> SSLISKTIKYDPAKDKLITLASGSFWGTEHMYRKYLNDRIVDSKVGYANGEESKKDSPSSVSYKRVSGGDTDFAEVLQVSYNPKVITLRELTDFFFRIHDPTTSNSQGPDKGTQYRSGLFAHSDADLKELAKIKEEWQPKWGNKIATVIEPIKNFYDAEEYHQLYLDKNPQGYACPTH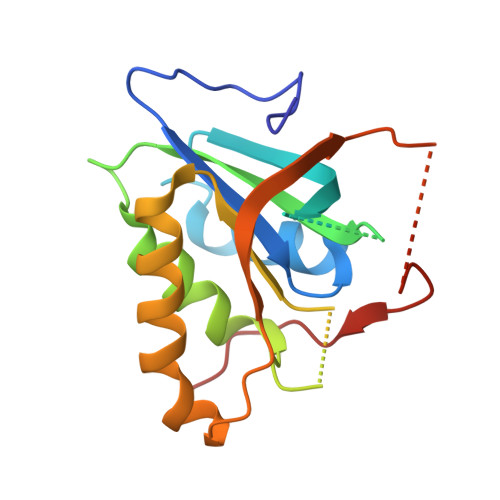YLREM>[2x]MSLLLCDIGNSNANFLDDNKYFTLNIDQFLEFKNEQKIFYINVNEHLKEHLKNQKNFINLEPYFLFDTIYQGLGIDRIAACYTIED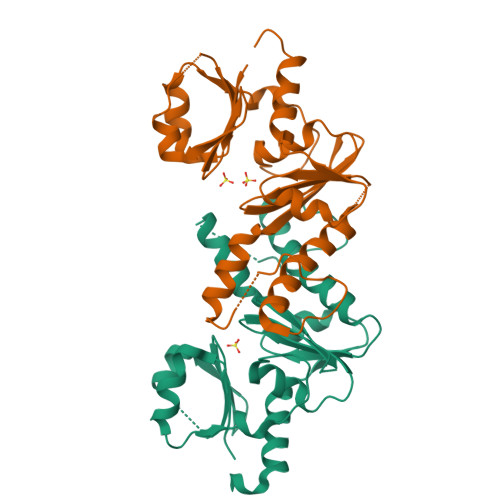GVVVDAGSAITIDIISNSIHLGGFILPGIANYKKIYSHISPRLKSEFNTQVSLDAFPQKTMDALSYGVFKGIYLLIKDAAQNKKLYFTGGDGQFLANYFDHAIYDKLLIFRGMKKIIKENPNLLYEGHHHHHH AvaII from the filamentous cyanobacterium Anabaena variabilis has attracted our interest because it exhibits robust activity against the RNA and DNA strands of an RNA/DNA heteroduplex. As most other enzymes with such properties, AvaII is a Type II restriction endonuclease predicted to belong to the PD-(D/E)XK superfamily. The enzyme is specific for DNA with the G↓GWCC sequence (where W stands for an A or T base of a ‘weak’ base pair) and cleaves it to products with three nucleotide long 5′-overhangs. The core of the AvaII protomer adopts the same conformation in all three structures, and consists of the characteristic αββββ motif of the PD-(D/E)XK endonucleases.

AvaII was prepared for crystallization in the presence of 5 mM Ca2+ ions. An ‘open’ conformation of the AvaII dimer is observed in the absence of nucleic acids and in complex with the RNA/DNA heteroduplex. In this form, the AvaII central channel is too wide for base-specific interactions with the bound oligoduplex and the enzyme only contacts the phosphodiester backbone. In the absence of nucleic acids a second protein dimer fills in the space between the protomers that should be occupied by the DNA double helix. The two open forms (in the absence of nucleic acids and in the scanning complex with the RNA/DNA duplex) are almost identical and no dynamic motions are found between them according to the DynDom server.

>[4x]MGSKFIQNAAEIAKKAMDSVDPSLSEKFTIVIRFLTDNPDAASALKGKERSIVGTEEYIIASATNFKKGRDPRTPLPPSTIPDEMVSVILNKYFEVPSEELEKAEEWHRLSMGAENIVGDLLERYIAEVIEPHGWIWCSGSMVRAVDFIYCDSENVWQSLQVKNRDNTENSSSAAIRHGTPIKKWFRTFSKKRGDNWDKFPSLEGKENLSEKGFKLYVEKYLSALRAIKALEHHHHHH>[2x]VETISFSFSEFEPGNDNLTLQGAALITQSGVLQLTKINQNGMPA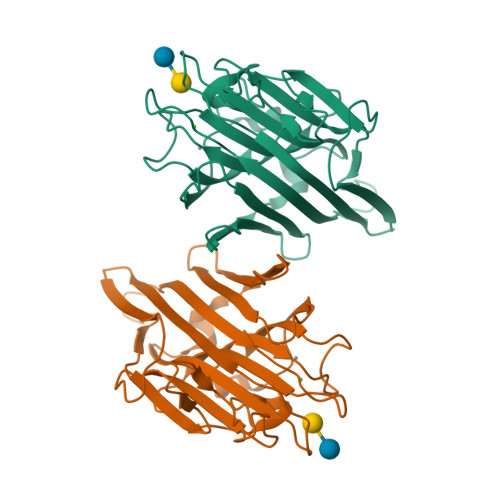WDSTGRTLYAKPVHIWDMTTGTVASFETRFSFSIEQPYTRPLPADGLVFFMGPTKSKPAQGYGYLGIFNNSKQDNSYQTLGVEFDTFSNPWDPPQVPHIGIDVNSIRSIKTQPFQLDNGQVANVVIKYDASSKILHAVLVYPSSGAIYTIAEIVDVKQVLPEWVDVGLSGATGAQRDAAETHDVYSWSFQASLPETNDAVIPTSNHNTFAI>AMATSTTPTILPALAAGLARGNIRVVDLTQTLSPSFPTLQLPSQFGQVQPFKIERISHYDASGPAWYWNNFSCGEHTGTHFDAPAHWITGRDYPGNSVDTIAPENFVAPAVVIDASAQVRENEDWLLTVDFLQAWEQRHGRIPAGAWVLF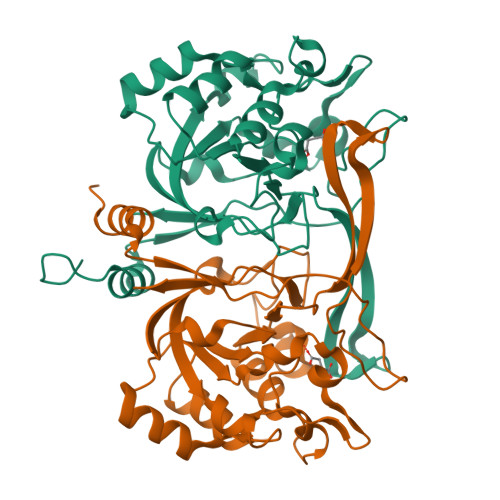RTDWSLRVGDAAAFLNIREDGAHTPGPTQEAVEWLIGERNVHGFGVETINTDAGQSYAWPLAYPCHTLMHGANRYGLQCLKNLDQLPPRGAFILAAPLKIEGGSGSPLRVLALVE[10x]In black-grass, upregulation of a phi (F)-class GST1 (AmGSTF1) has been shown to be a functional biomarker of MHR. Recombinant AmGSTF1 has been shown to exhibit both glutathione-S-transferase activity toward xenobiotics, as well as acting as a GPOX, reducing fatty-acid hydroperoxides to less reactive monohydroxy derivatives. The Phi (F) class GSTs, of which AmGSTF1 is an example, are found in all higher plants, being homodimeric enzymes in which each protomer of approximately 23–30 kDa with the catalytic serine residues located at the interface. Each protomer has two distinct domains; the N-terminal domain adopts the typical thioredoxin-fold, with the C-terminal domain being a bundle of at least five helices as demonstrated by the crystal structures of AmGSTF1 presented here.

In spite of extensive crystallisation and soaking efforts, no crystal with any substrate bound or any alternative crystal packing forms of the wild-type protein were obtained. Based on a careful analysis of the crystal packing, the key hydrophobic contact stabilising a crystallographic dimer interface shown in Fig. 1b was identified and three protein variants were designed to facilitate alternative packing. The core structure was found to be virtually identical to that of the native protein. However, the previously disordered loops in wild-type AmGSTF1 were now well-defined in the Phe112Thr variant and, for the first time, a glutathione molecule was determined as being bound in the G-site, confirming the validity of the design strategy. The Phe122Tyr variant therefore adopted the closed conformation for the two loops over the binding cleft with glutathione bound in the G-site.

> MAPVKVFGPAMSTNVARVTLCLEEVGAEYEVVNIDFNTMEHKSPEHLARNPFGQIPAFQDGDLLLWESRAISKYVLRKYKTDEVDLLRESNLEEAAMVDVWTEVDAHTYNPALSPIVYQCLTNPMMRGLPTDEKVVAESLEKLKKVLEVYEARLSKHSYLAGDFVSFADLNHFPYTFYFMATPHAALFDSYPHVKAWWDRLMARPAVKKIAATMVPPKA> AESLPDLKIEKLDEGVYVHTSFEEVNGWGVVPKHGLVVLVNAEAYLIDTPFTAKDTEKLVTWFVERGYKIKGSISSHFHSDSTGGIEWLNSRSIPTYASELTNELLKKDGKVQATNSFSGVNYWLVKNKIEVFYPGPGHTPDNVVVWLPERKILFGGGFIKPYGLGNLGDANIEAWPKSAKLLKSKYGKAKLVVPSHSEVGDASLLK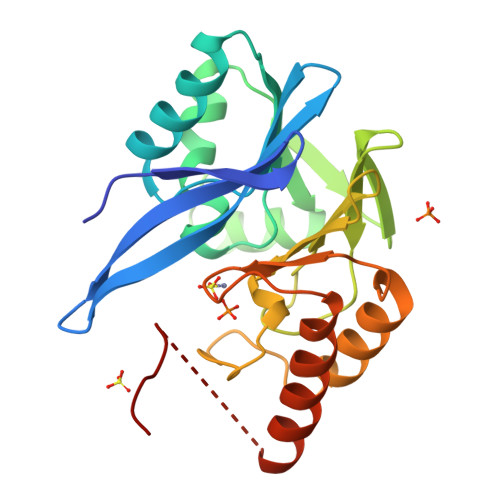LTLEQAVKGLNESKKPSKPSNWSHPQFEK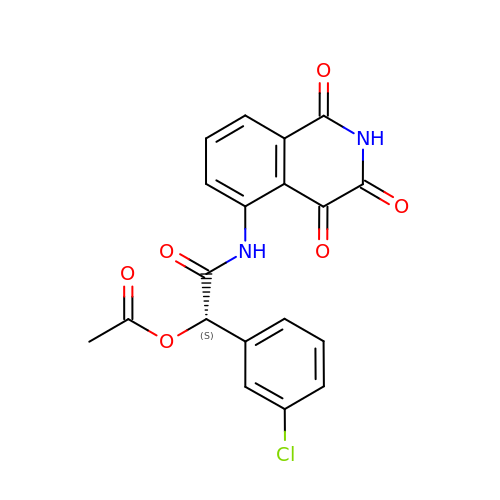(1S)-1-(3-chlorophenyl)-2-oxo-2-[(1,3,4-trioxo-1,2,3,4-tetrahydroisoquinolin-5-yl)amino]ethyl acetate | C19 H13 Cl N2 O6 | OVSAMUIBGQSLDC-INIZCTEOSA-N>[2x]ALFGSNDVTTAHSDYEIVLEGGSSSWGKVKARAKVNAPPASPLLPADADVKLNVKPLDPAKGFVRISAVFESIVDSTKNKLTIEADIANETKERRISVGEGMVSVGDFSHTFSFEGSVVNLFYYRSDAVRRNVPNPIYMQGRQFHDILMKVPLD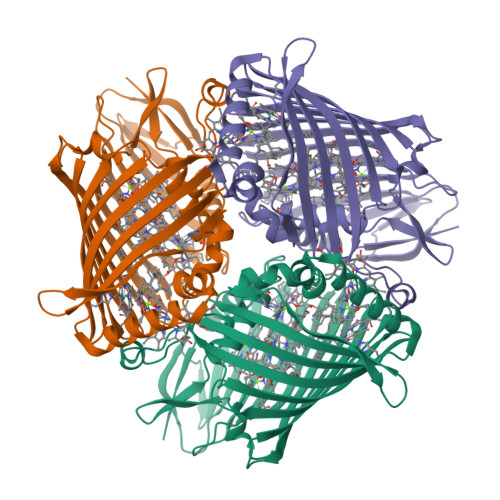NNDLIDTWEGTVKAIGSTGAFNDWIRDFWFIGPAFTALNEGGQRISRIEVNGLNTESGPKGPVGVSRWRFSHGGSGMVDSISRWAELFPSDKLNRPAQVEAGFRSDSQGIEVKVDGEFPGVSVDAGGGLRRILNHPLIPLVHHGMVGKFNNFNVDAQLKVVLPKGYKIRYAAPQYRSQNLEEYRWSGGAYARWVEHVAKGGVGQFEILYAQ>MLKAVILIGGPQKGTRFRPLSFEVPKPLFPVAGVPMIQHHIEACAQVPGMQEILLIGFYQPDEPLTQFLEAAQQEFNLPVRYLQEFAPLGTGGGLYHFRDQILAGSPEAFFVLNADVCSDFPLSAMLEAHRRQRHPFLLLGTTANRTQSLNYGCIVENPQTHEVLHYVEKPSTFISDIINCGIYLFSPEALKPLRDVFQRNQQDGQLEDSPGLWPGAGTIRLEQDVFSALAGQGQIYVHLTDGIWSQIKSAGSALYASRLYLSRYQDTHPERLAKHTPGGPWIRGNVYIHPTAKVAPSAVLGPNVSIGKGVTVGEGVRLRESIVLHGATLQEHTCVLHSIVGWGSTVGRWARVEGTPSDPNPNDPRARMDSESLFKDGKLLPAITILGCRVRIPAEVLILNSIVLPHKELSRSFTNQIIL[4x];>MKALILVGGYGTRLRPLTLSTPKPLVDFCNKPILLHQVEALAAAGVDHVILAVSYMSQVLEKEMKAQEQRLGIRISMSHEEEPLGTAGPLALARDLLSETADPFFVLNSDVICDFPFQAMVQFHRHHGQEGSILVTKVEEPSKYGVVVCEADTGRIHRFVEKPQVFVSNKINAGMYILSPAVLQRIQLQPTSIEKEVFPIMAKEGQLYAMELQGFWMDIGQPKDFLTGMCLFLQSLRQKQPERLCSGPGIVGNVLVDPSARIGQNCSIGPNVSLGPGVVVEDGVCIRRCTVLRDARI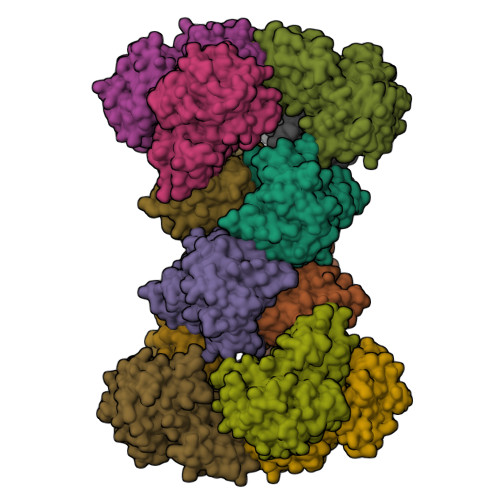RSHSWLESCIVGWRCRVGQWVRMENVTVLGEDVIVNDELYLNGASVLPHKSIGESVPEPRIIM[8x]>MRNDGGFLDWWEDLRSEMQSITDSQEVFAVLEKEVRRLGFDYYAYCVRHPIPFTRPRIFMFGNYPPAWQEHYQAQNYFAIDPTIRHCLRSGNHIVWSDDLFADAQELWDDARDYGLRHGATHSCMAPNG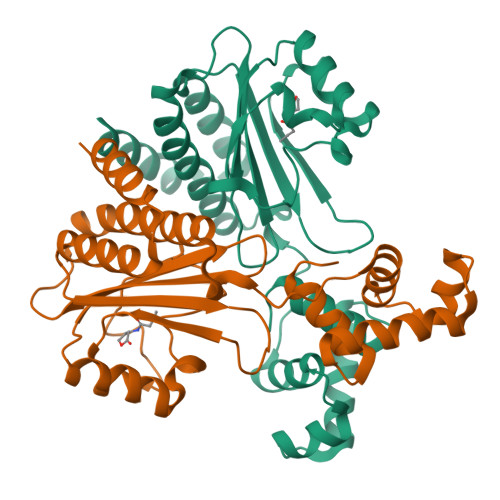VMGFLSVARSSPAISPHEREELRLRMRCLIELLHQTLTELNHPSLQPQPICLSKREREILRWTADGKTSAEIAKILGISESTVNFHLKNIQKKFNAPNKTQAAAYAAALGLI[4x]> HMGAPATVTEQGEDITSKKDRGVLKIVKRVGNGEETPMIGDKVYVHYKGKLSNGKKFDSSHDRNEPFVFSLGKGQVIKAWDIGVATMKKGE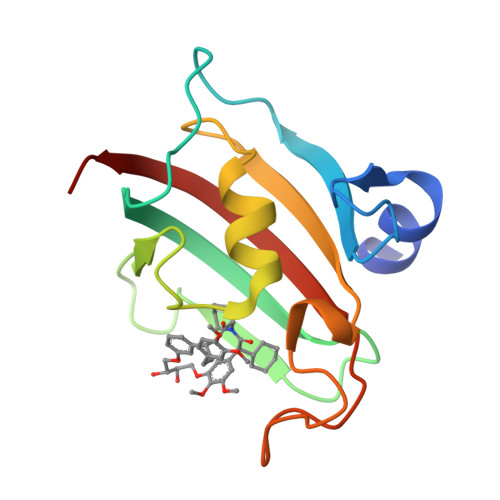IAHLLIKPEYAYGSAGSLPKIPSNATLFFEIELLDFKGE> DENSGKSQTVIV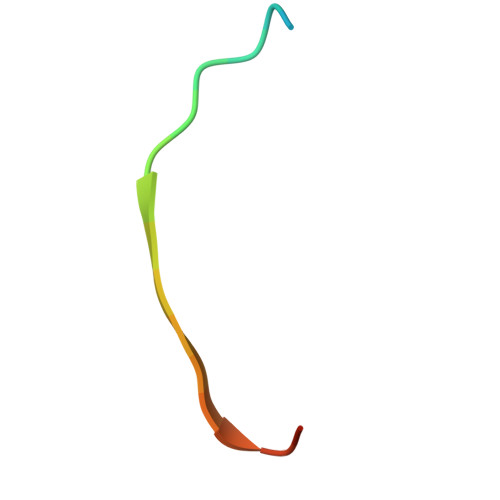GPWGAKVS> MAKQYDSVECPFCDEVSKYEKLAKIGQGTFGEVFKARHRKTGQKVALKKVLMENEKEGFPITALREIKILQLLKHENVVNLIEICRTKASPYNRCKGSIYLVFDFCEHDLAGLLSNVLVKFTLSEIKRVMQMLLNGLYYIHRNKILHRDMKAANVLITRDGVLKLADFGLARAFSLAKNSQPNRYTNRVVTLWYRPPELLLGERDYGPPIDLWGAGCIMAEMWTRSPIMQGNTEQHQLALISQLCGSITPEVWPNVDNYELYE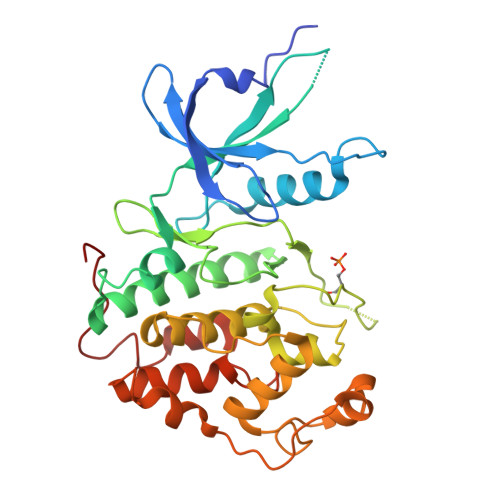KLELVKGQKRKVKDRLKAYVRDPYALDLIDKLLVLDPAQRIDSDDALNHDFFWSDPMPSDLKG> MSETSASYYQDLANKESANYNNAISQKAAIDAQISRLETAKTNLSTQINNFQTDIVDKMSDIEGEDSSQFKGD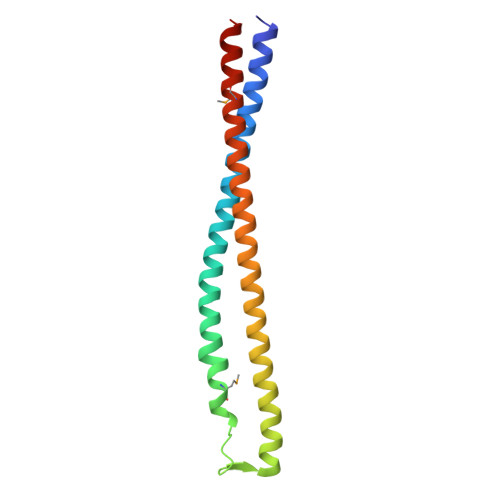RKTKYAEQYTSTKSAATTNKTSHDTNLTSITNKITELQTQSTSLQSAADTAYSNMLSYQASANAANTE> GPKPKNTKENLSKSSWRQEWLANLKLISVSLVDEFPSELSDSDRQIINEKMQLLKDIFANNLKSAISNNFRESDIIILKGEIEDYPMSSEI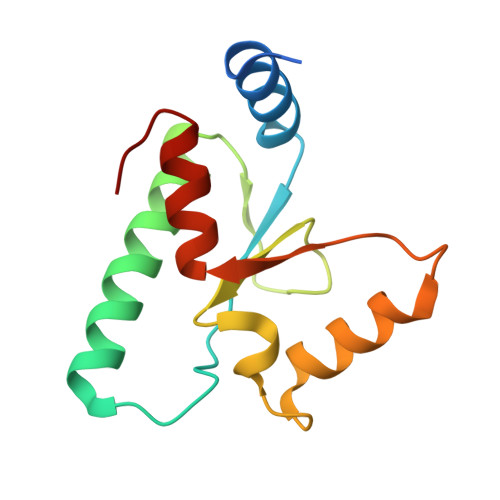KIYYNELQNKPDAKKARFWSFMKTQRFVSNMGFDIQ> QKKRFLPQSVLIKREDEIAFDDFHLDARK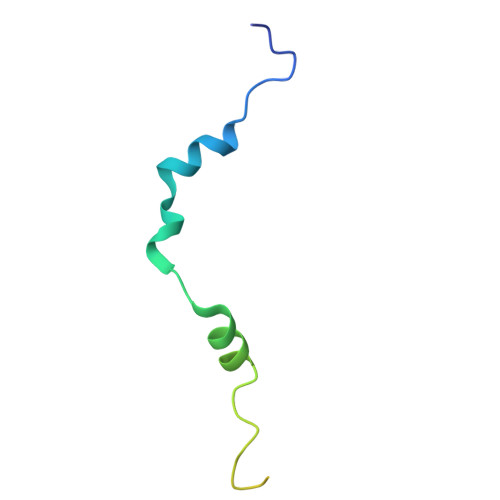VLNDLSATSENPFSSSPNTKKIKSKGKTLEVVPKKKNKKII> MDGAGAEEVLAPLRLAVRQQGDLVRKLKEDKAPQVDVDKAVAELKARKRVLEAKELALQPKDDIVDRAKMEDTLKRRFFYDQAFAIYGGVSGLYDFGPVGCALKNNIIQTWRQHFIQEEQILEIDCTMLTPEPVLKTSGHVDKFADFMVKDVKNGECFRADHLLKAHLQKLMSDKKCSVEKKSEMESVLAQLDNYGQQELADLFVNYNVKSPITGNDLSPPVSFNLMFKTFIGPGGNMPGYLRPETAQGIFLNFKRLLEFNQGKLPFAAAQIGNSFRNEISPRSGLIRVREFTMAEIEHFVDPSEKDHPKFQNVADLHLYLYSAKAQVSGQSARKMRLGDAVEQGVINNTVLGYFIGRIYLYLTKVGISPDKL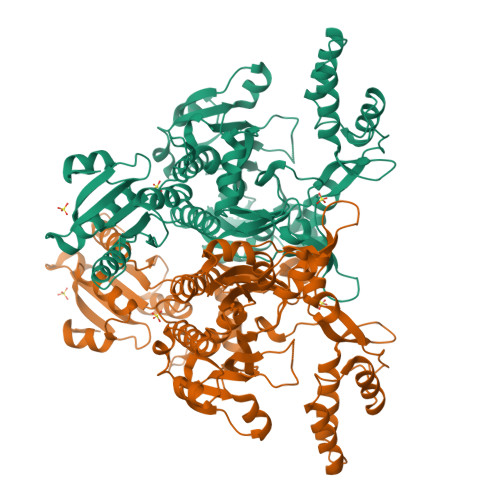RFRQHMENEMAHYACDCWDAESKTSYGWIEIVGCADRSCYDLSCHARATKVPLVAEKPLKEPKTVNVVQFEPSKGAIGKAYKKDAKLVMEYLAICDECYITEMEMLLNEKGEFTIETEGKTFQLTKDMINVKRFQKTLYVEEVVPNVIEPSFGLGRIMYTVFEHTFHVREGDEQRTFFSFPAVVAPFKCSVLPLSQNQEFMPFVKELLEALTRHGVSHKVDDSSGSIGRRYARTDEIGVAFGVTIDFDTVNKTPHTATLRDRDSMRQIRAEISELPSIVQDLANGNITWADVEARYPLFEGQETGKKETIEEHHHHHH> GAMSTGAVVTESQTYKKRADFLSNDDYAVY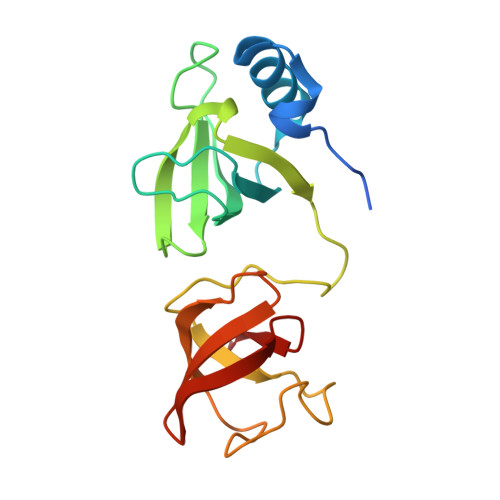VRENIQVGMMVRCCRAYEEVCEGDVGKVIKLDRDGLHDLNVQCDWQQKGGTYWVRYIHVELIGYPPPSSSSHIKIGDKVRVKASVTTPKYKWGSVTHQSVGVVKAFSANGKDIIVDFPQQSHWTGLLSEMELVP> GSSPVQSGFNNGTISNYMYFERRPDLLTKGTQDKAAAVKLKIENFYQSSVKYAIERNERRVELETELTSHNWSEERKSRQLSSLGKKESQFLRLRRTRLSLEDFHTVKVIGKGAFGEVRLVQKKDTGKIYAMKTLLKSEMYKKDQLAHVKAERDVLAGSDSPWVVSLYYSFQDAQYLYLIMEFLPGGDLMTMLIRWQLFTEDVTRFYMAECILAIETIHKLGFIHRAIKPDNILIDIRGHIKLSDFGLSTGFHKTHDSNYYKKLLQQDEATNGISKPGTYNANTTDTANKRQTMVVDSISLTMSNRQQIQTWRKSRRLMAYSTVGTPDYIAPEIFLYQGYGQECDWWSLGAIMYECLIGWPPF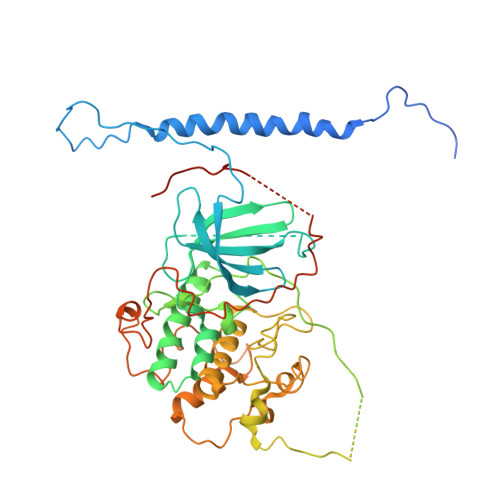CSETPQETYRKIMNFEQTLQFPDDIHISYEAEDLIRRLLTHADQRLGRHGGADEIKSHPFFRGVDWNTIRQVEAPYIPKLSSITDTRFFPTDELENVPDSPAMAQAAKQREQMTKQGGSAPVKEDLPFIGYEYSRFDYLTRKNAL>[2x]MPDDAKTANTTTAATTKNAENNRITPVTVIGLGAMGRALAGALLDAGYPTTVWNRTAGRGEDLVARGATLAASPAEAVRAGEVVLVCVVDYAASQAILEPVAADLA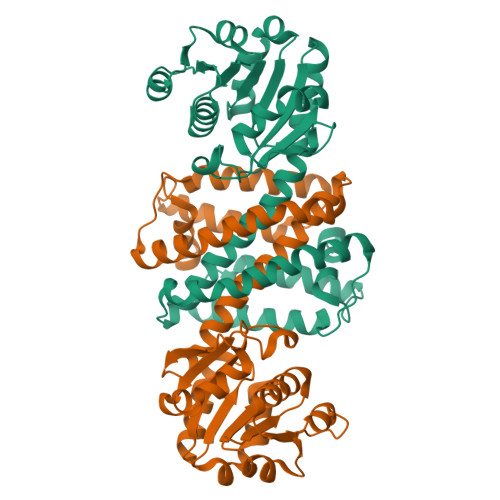GRVLVNVTSDSPERAREAAKWADGHGIRYLDGAVMIPTVMVGSTDALLFYAGDKSAYDEHEQVFTSLGGQSAYVGADHGLAAVYDLSMLDFFWTSMSGLVHGYALAAKDGVPATSIAPFLKAHISLLSLLIEVTAKDLDAGEYPGAEGNLAMEVEGIEHILHAAELRGLDVSVLRSVRDVARRAVDLGHGADSWSATVEGARNPA> SNAGGSATGTGLVYVDAFTRFHCLWDASHPECPARVSTVMEMLETEGLLGRCVQVEARAVTEDELLLVHTKEYVELMKSTQNMTEEELKTLAEKYDSVYLH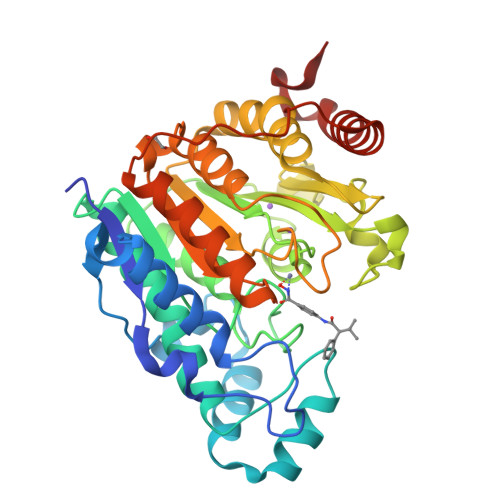PGFFSSACLSVGSVLQLVDKVMTSQLRNGFSINRPPGHHAQADKMNGFCMFNNLAIAARYAQKRHRVQRVLIVDWDVHHGQGIQYIFEEDPSVLYFSVHRYEDGSFWPHLKESDSSSVGSGAGQGYNINLPWNKVGMESGDYITAFQQLLLPVAYEFQPQLVLVAAGFDAVIGDPKGGMQVSPECFSILTHMLKGVAQGRLVLALEGGFNLQSTAEGVCASMRSLLGDPCPHLPSSGAPCESALKSISKTISDLYPFWKSLQTFE>[2x]MLVFIDDGSTNIKLQWQESDGTIKQHISPNSFKREWAVSFGDKKVFNYTLNGEQYSFDPISPDAVVTTNIAWQYSDVNVVAVHHALLTSGLPVSEVDIVCTLPLTEYYDRNNQPNTENIERKKANFRKKITLNGGDTFTIKDVKVMPESIPAGYEVLQELDELDSLLIIDLGGTTLDISQVMGKLSGISKIYGDSSLGVSLVTSAVKDALSLARTKGSSYLADDIIIHR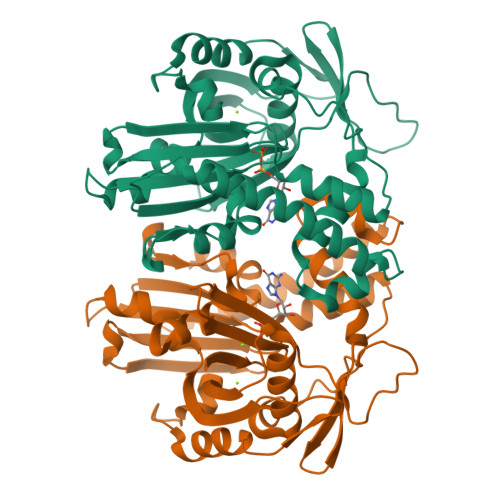KDNNYLKQRINDENKISIVTEAMNEALRKLEQRVLNTLNEFSGYTHVMVIGGGAELICDAVKKHTQIRDERFFKTNNSQYDLVNGMYLIGN> MTLETTLFPLEGLEGLTASYQLYAVKGLSGLDETEYHKNVNLLVRRLSFSMKAPFVALSRDGEQFIAVPNYVTEFPVDHRVVRAMVKLVPTGEPLNLRFDAADDEYDGLRLRYLDFVLQQPLFANHH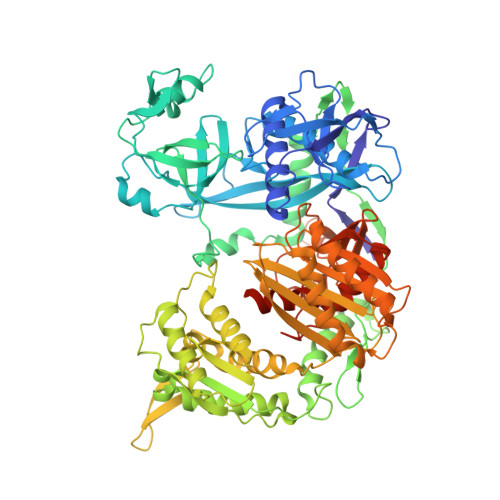LWQPGSGQPFFHKKPLKRLDDVDLYDGVSVRAAKHPEGGFGIVCDARSKFITHTPIGARADRKRLGKLINRSCLYKMGDHWYQFRIDAVSDWKVGEPSLFEGNVPISLAQQLVRTAGNAAPKSIIDLDPEGGALEYFTSTNERRMAPAELCFLIEDTHGRRAAKLQRQTILSPSERRARVNGFIRRYLSELNIGGAKLSAGARAHAFFTETHMPPALSFGNGTVLAPDTSKDRFQAMQEYSSMRRTMMLDKKVGFFHQDVFPPQTLLLPESVKKSWGPAFASDFVGTVQELYPAGGYRPEIIEYRDKAYGGGVPGQMKALLEVAERGEIKSGDVLVMLHRINGAPRAQDKLAAMVCNEFEKRFGKRVQVIHSDSPGRGYKRIFKNDKPTYVQQRGRGVNIKGYLKGAALNKVCLGNSRWPFVLRDPLNADVTIGIDVKNNMAVFTMVAEGGRIVRVQRSRSRQREQLLESQVTQVITEMLSKELPEIKKQVQRVVIHRDGRAWPAEIAGARKTFADMAESGLIAVDADVSVFEVLKSSPAPLRLFSFEEPTQENPKGVINPVLGSWLKLSENDGYICTTGAPLLLQGTADPLHVRKAFGPMAIEDALKDVFDLSCLTWPKPDSCMRLPLTIKLCDIALFDDAAEYDVDVVRFADGNTGEASA In 2018, two novel influenza-like virus genomes were detected from the lungs of amphibian-Wuhan Asiatic toad (Bufo gargarizans) and the gill samples of ray finned fish-Wuhan spiny eel (Mastacembelus aculeatus), respectively. The HA of the Asiatic toad influenza-like virus (tHA) and spiny eel influenza-like virus (eHA) share 23.0% and 42.8% amino acid sequences homology with IBV HA, respectively. It was revealed that eHA could bind to monosialic ganglioside 2 (GM2) and mediates fusogenicity under various pH conditions. The tHA and eHA resembles the typical homotrimeric conformation.

To elucidate the molecular mechanism, the cryo-EM structures of the extracellular domain of apo-tHA and apo-eHA were determined at resolutions of 2.65 Å and 2.95 Å, respectively. While the amino acid sequence of eHA is only 42.8% identity to IBV HA, the overall structure of eHA is very similar to IBV HA, with an RMSD of 3 Å. In eHA, α-helix A and α-helix B are connected by an interhelical loop, similar to canonical HA. The overall packing of eHA is slightly looser than that of IAV and IBV, but more compact than that of tHA. For the eHA, the HA2 subunit of eHA exhibits significantly more intra-subunit interactions than HA1. Consequently, the structural integrity of the eHA trimer is likely maintained predominantly by the HA2 subunit. In eHA, the base of the groove is formed by N95, W158, W191 and Y202. Although there is a noticeable cavity at the RBS of eHA, this region exhibits a slight negative charge, which repels the negative charge of SA. Additionally, compared to IBV HA, the P238 in the 240-loop corresponds to T238 in eHA, and this change causes an outward shift in the 240-loop. Furthermore, we compared the RBS of all canonical IAV and IBV strains with that of eHA and found that only the 240-loop of eHA RBS is outward shift. These factors collectively contribute to eHA’s inability to bind to canonical SA receptors.

>[3x]DKICAGVASGKGTHRVETITKGEVLVTNAINMTHTPTSGPFGDLKTGNVRDKLCPTCTGCTDMDVALMTPTCNGVIPEAIAAIQHENRPLQSKCNPILHDLGNTRQLPNLLRKYKKIRKSSGIAFPLASYADQPVISNPSGNCRDGNGVESEFGSLLWLTGNTKGAITGETITITHQCNNDEVMVLVWGAWADLSATMNTIYGVTTPQTYVSNFPSGRFSMSPFLGNFPALAETEATTATGRIYLRMEVLESGQRGTIQYQRGFMGPGKFWCLSEPIPVVKGAVKTNGAVSDCLHEVYGGISKPTPFYTGNRGKSVGNCPKWVRKPLLVVNGTKARDSISTRGLFGAIAGFLEGGWDGMIAGWHGYSSTGDHGTKVAADLVSTQKAMDAITARINNMNKMTERAFSVTDSTMQEIQKEIKDLDKKIDDVRADETAAQIEMIVLLENENIINAEDEHVHALKQKLTKMLGPSAQDMGDGCFIVDHQCKEDCLREIVSGNYTPSKYGMDEFKSPIITGTV The CP folds into three jelly-roll β sandwiches. The B and C domains clustered at the 3-fold axis. The structural variability of CP subunits within a capsid was very low. GFLV and TRSV are both transmitted by Xiphinema nematodes.

of a GFLV-F13 particle is viewed down a viral 2-fold axis. 3-fold and 2-fold symmetry axes is 155, 137 and 123 Å. ligand-binding pocket at the surface of the GFLV-F13 capsid. be recognized by compounds of the nematode feeding apparatus. axes may constitute a ligand recognition site. surface of the protein capsid which may constitute a binding site for the vector.

>[60x]GLAGRGVIYIPKDCQANRYLGTLNIRDMISDFKGVQYEKWITAGLVMPTFKIVIRLPANAFTGLTWVMSFDAYNRITSRITASADPVYTLSVPHWLIHHKLGTFSCEIDYGELCGHAMWFKSTTFESPRLHFTCLTGNNKELAADWQAVVELYAELEEATSFLGKPTLVFDPGVFNGKFQFLTCPPIFFDLTAVTALRSAGLTLGQVPMVGTTKVYNLNSTLVSCVLGMGGTVRGRVHICAPIFYSIVLWVVSEWNGTTMDWNELFKYPGVYVEEDGSFEVKIRSPYHRTPARLLAGQSQRDMSSLNFYAIAGPIAPSGETAQLPIVVQIDEIVRPDLSLPSFEDDYFVWVDFSEFTLDKEEIEIGSRFFDFTSNTCRVSMGENPFAAMIACHGLHSGVLDLKLQWSLNTEFGKSSGSVTITKLVGDKAMGLDGPSHVFAIQKLEGTTELLVGNFAGANPNTRFSLYSRWMAIKLDQAKSIKVLRVLCKPRPGFSFYGRTSFPV> EAGGVFKLIANDGKADRMIMANDLLNDRIKSIMCLRAKQGFSDPTPTLVDIERTHILLINSHYKPFAAMGYEYQKTRPNTGNPTYNSTIQFSIPQFGDFFSDMVVHVQLAATSASAGTVPALPAFIGADDQVLTSTSVVSATENTTSGVYTLYTQSYVNQQGTTQTVAAAATNFVRYCEYPGLRLFKRVKFEVNGNPLDEYTALAAIMYNKFHVPDFKLTGWKRLIGQEVPVEAASNLVNIASTTPWGSPIVALSDVNGTAVTGSPVN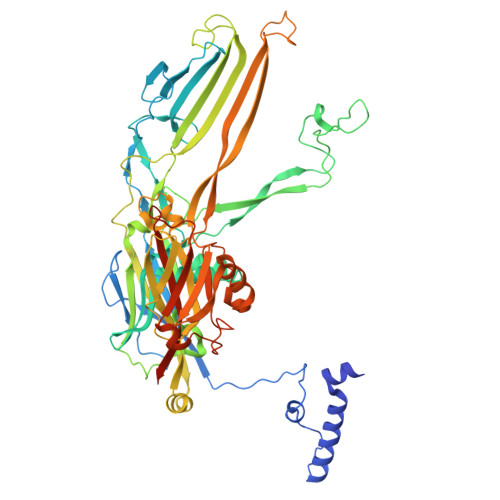AAITARKLTQVVFGAQTPKATQEQLNMFVPLLFWFRDPRLAIASVSIPYGQRFITVDIEQQSNILFTAPGNLFLQTTVETLLTTGAGKGTATGVLLTQYNRYTTYTPTLASGSSIDGTQAVQNIELYINNIFVTPEIHDIYIKRIGFTLIRVYREQVQREVNAADQVLQSQLKWPVEFIYLGLRPANNIAAGNTYQWRDWHHLTSVTNEPVYDVSQSYARVSIDDTVAPVGSTTFKQSASQVMQNQYIVPVETETLDTVRVKAHGIELYAQYRAQFYRDYIPWNYGSFNLVTPQDKGALFLNFCLYPGTYQPSGHVNISRAREFYIEYTSSFCDSSNPCDLISIAKCINFLLISDGSAVLRYSTKEFYLQCLILRCI N~2~-(1,1-dioxido-2,3-dihydro-1,2-benzothiazol-6-yl)-N~4~-ethyl-5-fluoro-N~4~-(1H-indazol-4-yl)pyrimidine-2,4-diamine 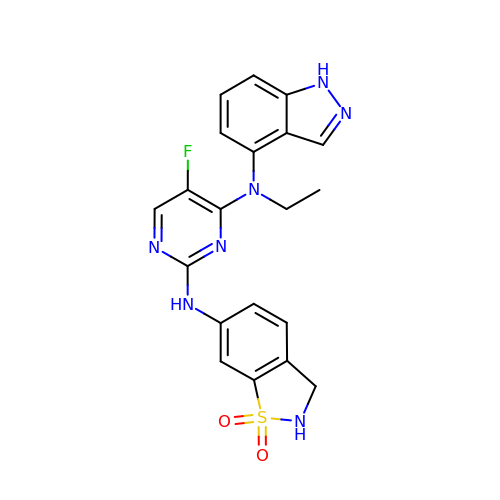| C20 H18 F N7 O2 S | LLBDUMUPBVPAMJ-UHFFFAOYSA-N>[2x]MENLGDKLSISQVYHLAQEYRDHAYSIANKIGSEEGLKQYYGLMNMSIQMFQLLKTKCTLSVLEDSKVTFEMVELLIQETYNFDLAELYISSLKERLQTHQSDTDLVEEIMRCEFLLLHDLPLMRDSKFHYKIALRNCNELVQYMVNLQDELYQNWASVFQYVGVMLCIKLKQHRRVKTSFHGLLSQCREKSQWKWFLNLCYVNYLLNERFPIPEDALQELRSTELHTVGPELYAWKLALEMVIQLCKDGNITDHLNEFKNFFDTNKQSLVTNEGKGCVIKIMPRIALKVELPMIFHYKELKNILLLLQSVSYIVNCYDEKGNFSRKFLPKVYSTTQKLIKNIAAGGVSMNELDSRIQTYKSILEFCEFYKVWEQTLLKGAVVTTESPKLGPSPGYVRLLQAMKVQFEGGGAVEEYTRLAQSGGTSSEVKMISLLNCYTVQAARVSRCSGDKQGELVEQCNKVWLQVEKLLQETDLQFNPIWECTVTILWLFSHFEPFSWNPLPCSDKQRAEYVSKLREFYSSNKFVAGEAVADNRFKLKKALLLQILVNYLGGRMLEHDLGEIYAISAKCFDMCRQQGGMRKVQYVIGIWHLMNCTVAMRGKDVALTNAKLEALVKQITSVKQ;>SNAMSYPGKDKNIPGRIIEALEDLPLSYLVPKDGLAALVNAPMRVSLPFDKTIFTSADDGRDVNINVLGTANSTTSSIKNEAEKERLVFKRPSNFTSSANSVDYVPTNFLEGLSPLAQSVLSTHKGLNDSINIEKKSEIVSRPEAKHKLESVTSNAGNLSFNDNSSNKKTKTSTGVTMTQANLA[2x];>[2x]MDFTSD

A separate and broadly conserved two-protein complex called Scc2/4 in yeast and NIPBL/Mau2 in humans loads cohesin onto chromosomes (Ciosk et al., 2000). We show that phosphorylation of the Ctf19 kinetochore protein by a conserved kinase, DDK, provides a binding site for the Scc2/4 cohesin loading complex, thereby directing cohesin loading to centromeres. Phosphorylated Ctf19 interacts directly with the previously identified conserved surface of Scc4, explaining both the requirement for DDK in centromeric cohesion establishment and the nature of Scc4-mediated targeting of cohesin loading to centromeres. We have shown previously that Scc2 recruitment to centromeres requires a conserved surface on the Scc4 protein (Hinshaw et al., 2015).

To observe the interaction between phosphorylated Ctf19 and Scc4 directly, we determined the crystal structure of a phosphorylated Ctf19 N-terminal peptide (MDFpTpSD) bound to Scc21–181-Scc4. Iterative density modification with non-crystallographic symmetry averaging revealed extra density near the Scc4 conserved patch, allowing us to model key Ctf19 residues, including the conserved F3 and the phosphorylated T4 and S5 residues. The phosphorylated Ctf19 residues T4 and S5 make electrostatic contacts with lysine side chains protruding from the Scc4 surface required for centromere cohesion (Scc4 K331 and K267). Coordination of these phosphates traps Ctf19 F3 between two aromatic side chains deep within the Scc4 conserved pocket (Scc4 F328 and F263). The structure also explains why the scc4-m3, scc4-m35, and scc4-m7 alleles abrogate Scc2 targeting to centromeres (Hinshaw et al., 2015). The conserved residues F324 and K331 are mutated in all three alleles. In addition to direct coordination of the phosphate at Ctf19 T4 by Scc4 K331, residue F324 stabilizes the position of Scc4 F328 and therefore aids in recognition of Ctf19 F3. Scc4 residues Y298 and K299 were mutated in the scc4-m7 allele. Y298 helps coordinate the phosphate at Ctf19 S5, and K299 makes contact with the Ctf19 peptide backbone, explaining the contribution of these residues to the scc4-m7 allele. We found that Ctf191–6 phosphorylated at amino acid residues T4 and S5 bound Scc21–181-Scc4 in vitro, while an unphosphorylated peptide did not.2-[2-[1-[2-(3,4-dichlorophenyl)ethyl]azetidin-3-yl]oxyphenyl]-~{N}-(3-pyrrolidin-1-ylpropyl)pyridine-4-carboxamide 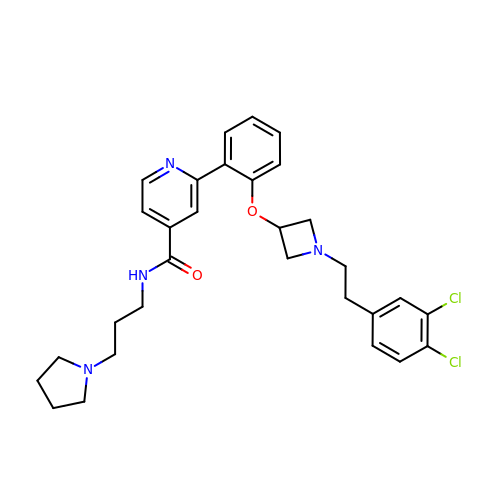| C30 H34 Cl2 N4 O2 | AGSYPSPYUHOIIZ-UHFFFAOYSA-N> GHKPEPTDEEWELIKTVTEAHVATNAQGSHWKQKRKFLPEDIGQAPIVNAPEGGKVDLEAFSHFTKIITPAITRVVDFAKKLPMFCELPCEDQIILLKGCCMEIMSLRAAVRYDPESETLTLNGE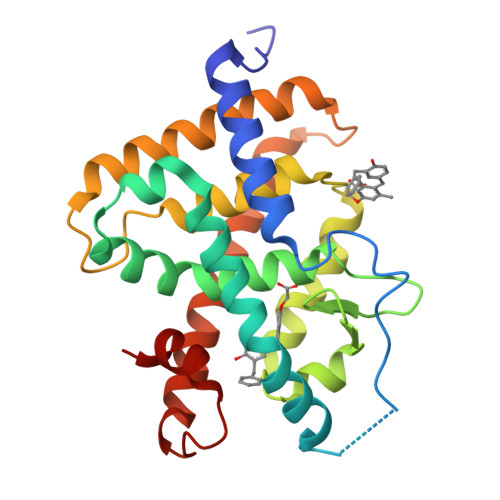MAVTRGQLKNGGLGVVSDAIFDLGMSLSSFNLDDTEVALLQAVLLMSSDRPGLACVERIEKYQDSFLLAFEHYINYRKHHVTHFWPKLLMKVTDLRMIGACHASRFLHMKVECPTELFPPLFLEVFED>[2x]MAKVSLEKDKIKFLLVEGVHQKALESLRAAGYTNIEFHKGALDDEQLKESIRDAHFIGLRSRTHLTEDVINAAEKLVAIGAFAIGTNQ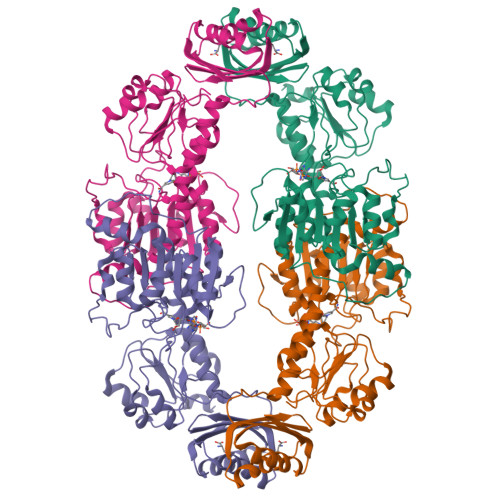VDLDAAAKRGIPVFNAPFSNTRSVAELVIGELLLLLRGVPEANAKAHRGVWNKLAAGSFEARGKKLGIIGYGHIGTQLGILAESLGMYVYFYDIENKLPLGNATQVQHLSDLLNMSDVVSLHVPENPSTKNMMGAKEISLMKPGSLLINASRGTVVDIPALADALASKHLAGAAIDVFPTEPATNSDPFTSPLAEFDNVLLTPHIGGSTQEAQENIGLEVAGKLIKYSDNGSTLSAVNFPEVSLPLHVGRRLMHIHENRPGVLTALNKIFAEQGVNIAAQYLQTSAQMGYVVIDIEADEDVAEKALQAMKAIPGTIRARLLY> MTLHSKSSQYRRLRTEWKNNVYLARSRIQGLGLYAAKDLEKHTMVIEYIGTIIRNEVANRREKIYEEQNRGIYMFRINNEHVIDATLTGGPARYINHSCAPNCVAEVVTFDKEDKIIIISSRRIPKGEELTYDYQFDFEDDQHEIP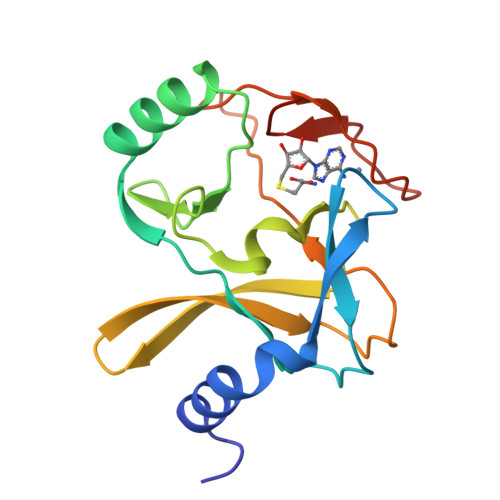CHCGAWNCRKWMKGHHHHHH> MSTKDLFAEPNLKQITVWARG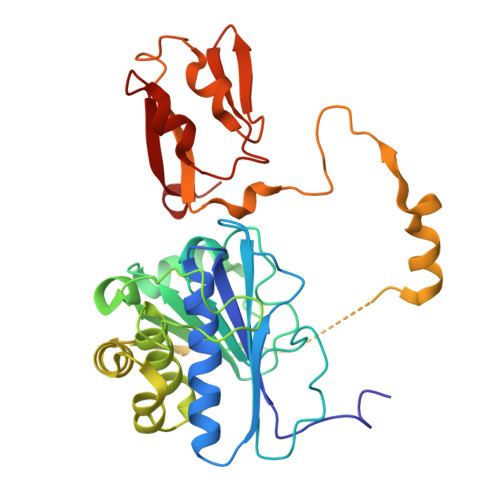VVMNKDARDIVVALTEAAAKEGKYVQAWENYVDLPDRIYVPVRAYARISSDPIESKYIYENETPDIVVLVEESLIKGVPILKGIRPGSTLVVNTKRSIDTILEFLGDTGNLAQIVTVDANSMAEAVMTLSGAEGATDATGIGAGIAAPIAGAVVKATGIVDVENLAAVVKNPAAMRRGYAEAQVRQLPPHEAVEEAAVSATELLRQMPFAGTVPSPVTENEGMVTGNWRIQRPIIDREACTECYTCWIYCPDSCITRTEEGPVFNMKYCKGCGLCTAVCPSGALTNVPELDFKD> RPRREALFFPSQVTCTEALLRAPGAELAELPEGCPCGLPHGESALSRLLRALLAARASLDLCLFAFSSPQLGRAVQLLHQRGVRVRVVTDCDYMALNGSQIGLLRKAGIQVRHDQDPGYMHHKFAIVDKRVLITGSLNWTTQAIQNNRENVLITEDDEYVRLFLEEFERIWEQFNPT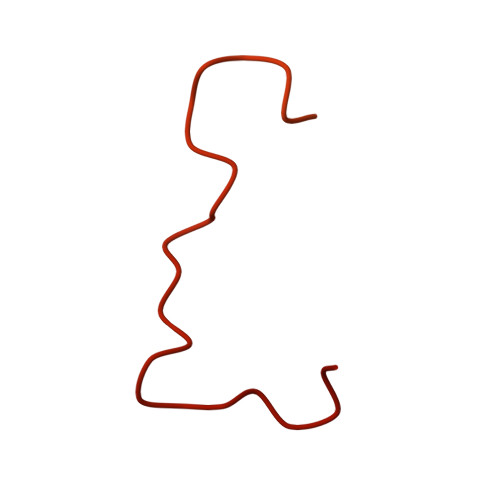KYTFFPPKKSHGSCAPPVSRAGGRLLS>MMTHEENELLCRVEGDAPMGRLMRRHWTPICLVEEVGEPDGTPVKARAFGEDLVVFRDSEGRVGVMDEYCPHRRASLVYGRNEEGGLRCLYHGWKMDVDGNVLEMASEPAASGMVDKVKHTAYPTQEWAGMVWAYMGPKETMPEFLPPAWAPTADTRVSIAKVLLPCNWAQILEGAIDSAHSSSLHSSDMVPARVDGAKATDKTWLRPSTDKAPRMQVQRTGYGFRYAALRRPLSNAAENDYVRSTVFVAPATALIPPNNLYNVANIN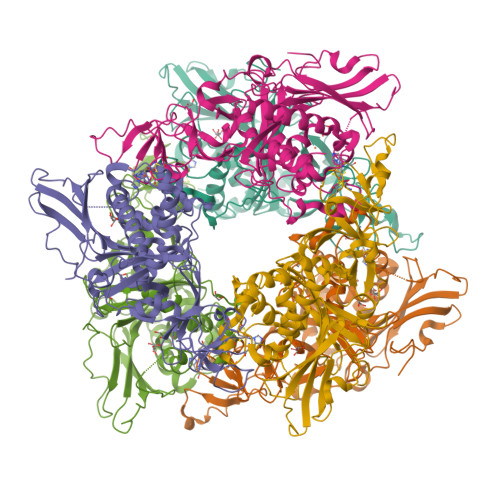VPMDDTNTAFYFIAWGHPSQTPETETWRKFLRQTVGVDLDQNYRPLRNEANKFWQDRNAMKAGNFTGITGFPNQDVAMWLTMGPIADRTHDRLGASDLAIVEFRKQMLDAVKAFEQGAPAIGTGVEAATPTVCSFQAIVPKTTDWRTYDAHYVWLDGQDRPEFEPSYSVKS[6x]>MGSDKIHHHHHHMEEKRLSAKKGLPPGTLVYTGKYREDFEIEVMNYSIEEFREFKTTDVESVLPFRDSSTPTWINITGIHRTDVVQRVGEFFGIHPLVLEDILNVHQRPKVEFFENYVFIVLKMFTYDKNLHELESEQVSLILTKNCVLMFQEKIGDVFDPVRERIRYNRGIIRKKRADYLLYSLIDALVDDYFVLLEKI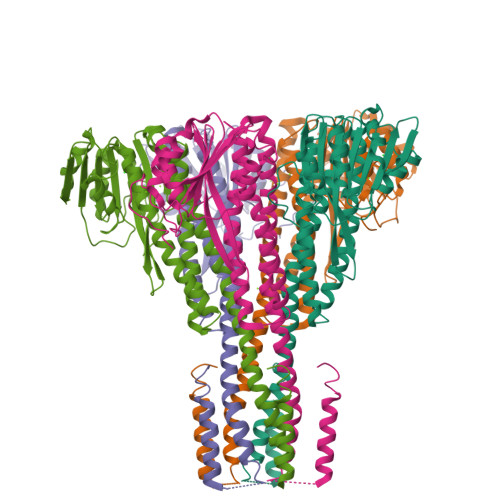DDEIDVLEEEVLERPEKETVQRTHQLKRNLVELRKTIWPLREVLSSLYRDVPPLIEKETVPYFRDVYDHTIQIADTVETFRDIVSGLLDVYLSSVSNKTNEVMKVLTIIATIFMPLTFIAGIYGMNFEYMPELRWKWGYPVVLAVMGVIAVIMVVYFKKKKWL[10x]> GLIVDTRDVEERVHVMRKTKLAPTVAHGVFNPEFGPAALSNKDSRLNEGVVLDEVIFSKHKGDTKMSAEDKALFRRCAADYASRLHSVLGTANAPLSIYEAIKGVDGLDAMEPDTAPGLPWALQGKRRGALIDFENGTVGPEVEAALKLMEKREYKFACQTFLKDEIRPMEKVRAGKTRIVDVLPVEHILYTRMMIGRFCAQMHSNNGPQIGSAVGCNPDVDWQRFGTHFAQYRNVWDVDYSAFDANHCSDAMNIMFEEVFRTEFGFHPNAEWILKTLVNTEHAYENKRITVEGGMPSGCSATSIINTILNNIYVLYALRRHYEGVELDT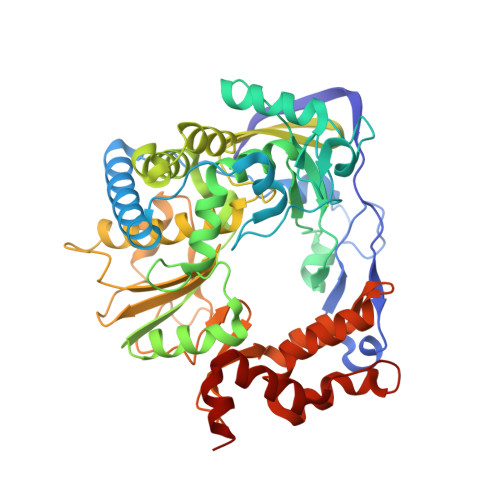YTMISYGDDIVVASDYDLDFEALKPHFKSLGQTITPADKSDKGFVLGHSITDVTFLKRHFHMDYGTGFYKPVMASKTLEAILSFARRGTIQEKLISVAGLAVHSGPDEYRRLFEPFQGLFEIPSYRSLYLRWVNAVCGDAAAAEHH> GRA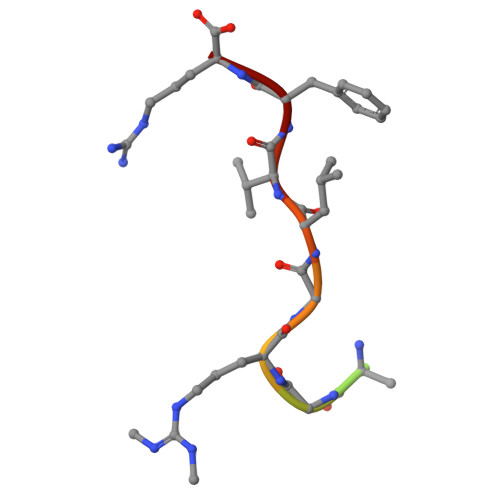GPAGRGLVFR> GSSQISDMTRDGLANKALAVARTLADSPEIRQGLQKKPQESGIQAIAEAVRKRNDLLFIVVTDMQSLRYSHPEAQRIGQPFKGDDILKALNGEENVAINRGFLAQALRVFTPIYDENHKQIGVVAIGLE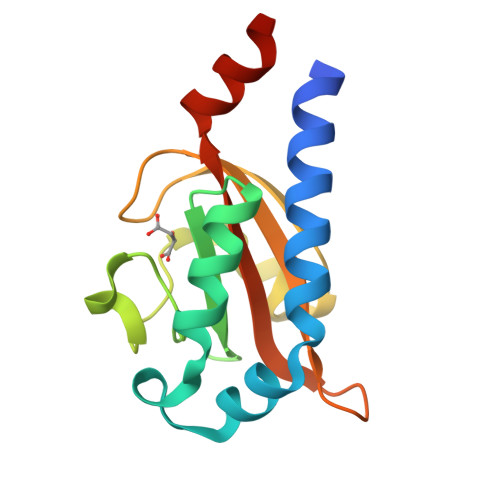LSRVTQQINDSRW> GPAMQDTVTKKGTGNFTAHGDIIHK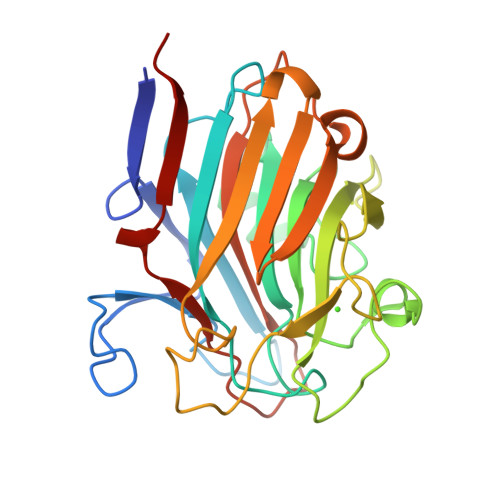TYKEEFPNEGTLTAFNTNFNPNTGTKGALEYNDKIDFNKDFTITVPVANNNQGNTTGADGWGFMFTQGNGQDFLNQGGILRDKGMANASGFKIDTAYNNVNDADKTNNLSQIGAAKVGYGTFVKNGADGVTNQVGQNALNTKDKPVNKIIYADNTTNHLDGQFHGQRLNDVVLNYDAATSTITATYAGKTWKATTDDLGIDKSQKYNFLITSSHMQNRYSNGIMRTNLEGVTITTPQAD> HGAWDEWSPWSLCSSTCGRGFRDRTRTCRPPQFGGNPCEGPE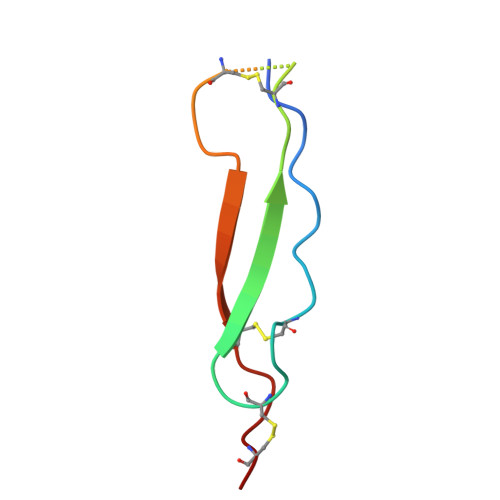KQTKFCNIALCP>MTPASYNLAVRRAAPAVVNVYNRGLNTNSHNQLEIRTLGSGVIMDQRGYIITNKHVINDADQIIVALQDGRVFEALLVGSDSLTDLAVLKINATGGLPTIPINARRVPHIGDVVLAIGNPYNLGQTITQGIISATGRIGLNPTGRQNFLQTDASINHGNSGGALVNSLGELMGINTLSFDKSNDGETPEGIGFAIPFQLATKIMDKLIRDGRVIRGYIGIGGREIAPLHAQGGGIDQLQGIVVNEVSPDGPAANAGIQVNDLIISVDNKPAISALETMDQVAEIRPGSVIPVVVMRDDKQLTLQVTIQEYPAT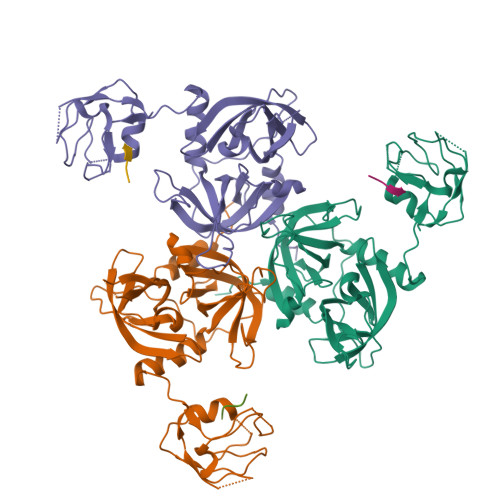N[3x];>DNRLGLVYWF[3x]> GSHMIEGYECQPIFLNVLEAIEPGVVCAGHDNNQPDSFAALLSSLNELGERQLVHVVKWAKALPGFRNLHVDDQMAVIQYSWMGLMVFAMGWRSFTNVNSRM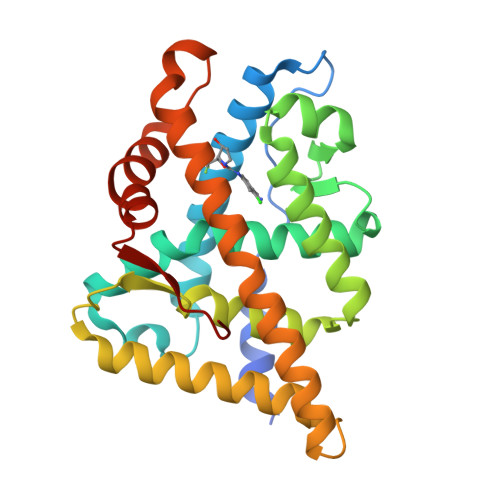LYFAPDLVFNEYRMHKSRMYSQCVRMRHLSQEFGWLQITPQEFLCMKALLLFSIIPVDGLKNQKFFDELRMNYIKELDRIIACKRKNPTSCSRRFYQLTKLLDSVQPIARELHQFTFDLLIKSHMVSVDFPEMMAEIISVQVPKILSGKVKPIYFHTQ> HIEGYECQPIFLNVLEAIEPGVVCAGHDNNQPDSFAALLSSLNELGERQLVHVVKWAKALPGFRNLHVDDQMAVIQYSWMGLMVFAMGWRSFTNVNSRMLYFAPDLVFNEYRMHKSRMYSQCVRMRHLSQEFGWLQITPQEFLCMKALL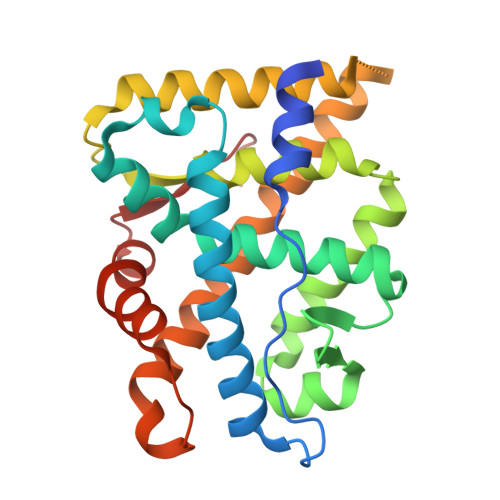LFSIIPVDGLKNQKFFDELRMNYIKELDRIIACKRKNPTSCSRRFYQLTKLLDSVQPIARELYQFTFDLLIKSHMVSVDFPEMMAEIISVQVPKILSGKVKPIYFHTQ N-methyl-N-(4,5,6,7-tetrahydro-1,3-benzothiazol-2-ylmethyl)prop-2-enamide 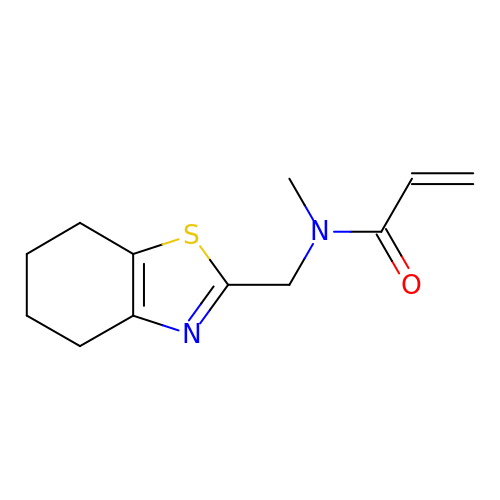| C12 H16 N2 O S | YJZOYCOTGFHVFV-UHFFFAOYSA-N> IVGGYTCGANTVPYQVSLNSGYHFCGGSLINSQWVVSAAHCYKSGIQVRLGEDNINVVEGNEQFISASKSIVHPSYNSNTLNNDIMLIKLKSAASLNSRVASISLPTSCASAGTQC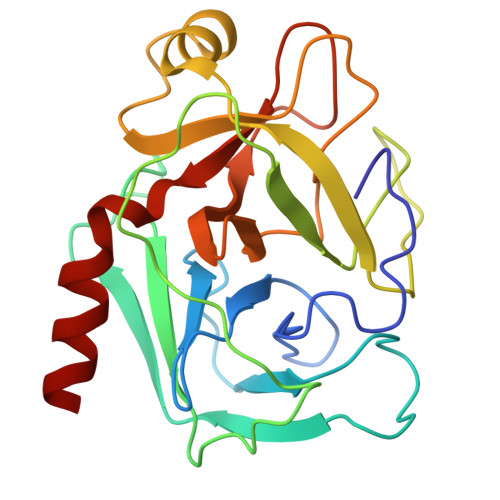LISGWGNTKSSGTSYPDVLKCLKAPILSDSSCKSAYPGQITSNMFCAGLEGGDSCQGDSGGPVVCSGKLQGIVSWGSGCAKNKPGVYTKVCNYVSWIKQTIASN> MRNRGFGRRELLVAMSMLVSVTGCARHASGARPASTTLPAGADLADRFAELERRYDARLGVYVPATGTTAAIEYRADERFAFCSTFKAPLVAAVLHQNPLTHLDKLITYTSDDIRSISPVAQQHVQTGMTIGQLCDAAIRYSDGTAANLLLADLGGPGGGTAAFTGYLRSLGDTVSRLDAEEPELNR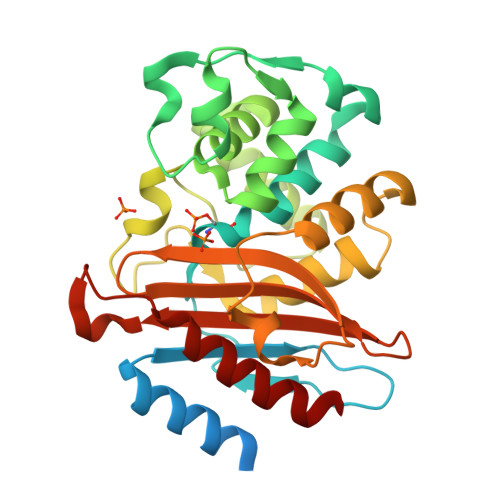DPPGDERDTTTPHAIALVLQQLVLGNALPPDKRALLTDWMARNTTGAKRIRAGFPADWKVIDKTGTGDYGRANDIAVVWSPTGVPYVVAVMSDRAGGGYDAEPREALLAEAATCVAGVLA> GRDYRTCLTIVQKLKKMVDKPTQRSVSNAATRVCRTGRSRWRDVCRNF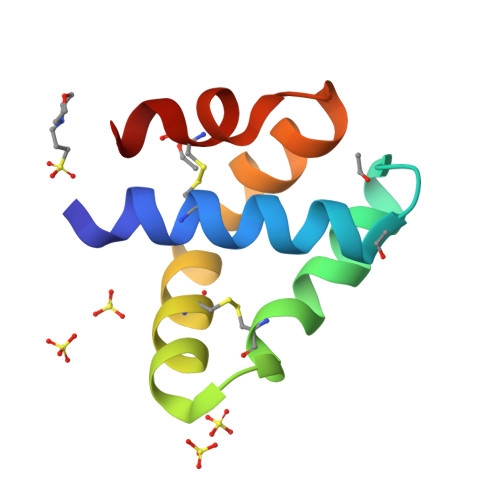MRRYQSRVIQGLVAGETAQQICEDLR>GARASVLSGGELDKWEKIRLRPGGKKQYKLKHIVWASRELERFAVNPGLLETSEGCRQILGRLQPSLQTGSEELRSLYNTIAVLYCVHQRIDVKDTKEALDKIEEEQNKSKKKAQQAAADTGNNSQVSQN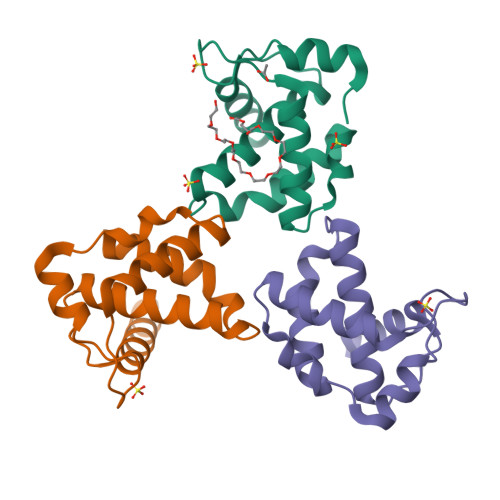YHHHHHH[6x]The A41 protein from VACV strain WR is a secreted 30 kDa glycoprotein and very similar proteins are expressed by camelpox virus, CPXV and all 16 strains of VACV tested. A41 is secreted from infected cells and has a primary amino acid sequence related to the vCCI family of poxvirus proteins that bind chemokines. Collectively these data show that A41 binds a subset of CC chemokines (CCL21, CCL25, CCL26 and CCL28) via a site that overlaps their GAG-binding site, but A41 does not inhibit leukocyte chemotaxis.

To understand the structural basis of the action of A41, its crystal structure was determined using protein expressed in E. coli and refolded from inclusion bodies. Phase determination was accomplished by MAD analysis of Seleno-methione (SeMet)-labelled crystals. Electron density was observed for residues 26–219 (numbering for mature protein begins at one) and the structure was refined to 1.9 Å (final R = 20.4 and Rfree = 25.2). A41 is a single domain protein with the distinctive β sandwich fold seen in the vCCI class of poxvirus chemokine binding proteins. Sheet I is largely buried from solvent by two long enveloping loops on one side and sheet II on the other (the other face of sheet II is exposed to solvent). One of these loops (the 9–11 loop, residues 113–144) wraps around the molecule and connects β strands 9 and 11, whilst the second comprises the C terminus and packs tightly against the face of sheet I, and bears strands 14 and 15. Eight cysteine residues in A41 form four disulphide bridges (C6-C166, C33-C199, C58-C104, and C112-C152). Despite sharing only 19% sequence identity with CPXV and ECTV vCCI, the structure of A41 is strikingly similar to the poxvirus vCCI family of secreted chemokine binding proteins. The surface charge properties of A41 are broadly similar to those seen in other poxvirus vCCI proteins, although sheet I exhibits a large patch of positive charge whereas in CPXV vCCI sheet I is comparatively uncharged. The absence of the 2–4 loop in A41 may explain the specificity of A41 for certain CC chemokines and underlies the weakness of the interaction.

> MAHHHHHHDDKSVCDSDNKEYMGIEVYVEATLDEPLRQTTCESKIHKYGASVSNGGLNISVDLLNCFLNFHTVGVYTNRDTVYAKFASLDPWTTEPINSMTHDDLVKLTEECIVDIYLKCEVDKTKDFMKTNGNRLKPRDFKTVPPSNVGSMIELQSDYCVNDVTTYVKIYDECGNIKQHSIPTLRDYFTTKNGQPRKILKKKFDNC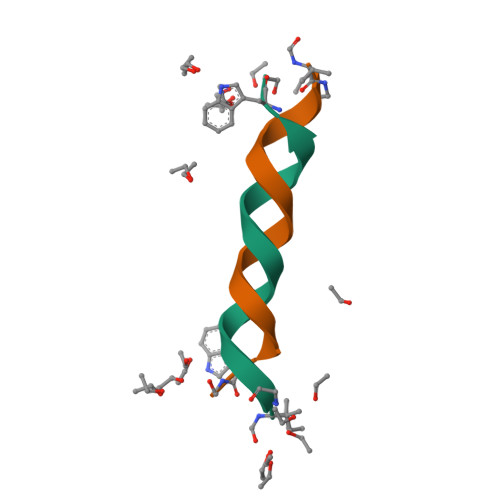> XGALAVVVWLYLWLWX;> VGALAVVVWLWLWLWX>[2x]MIDYTAAGFTLLQGAH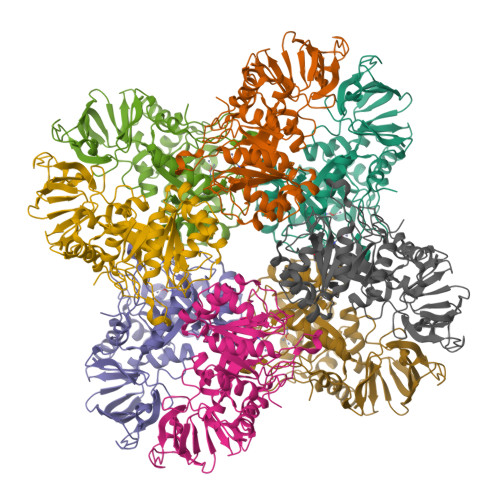LYAPEDRGICDVLVANGKIIAVASNIPSDIVPNCTVVDLSGQILCPGFIDQHVHLIGGGGQAGPTTRTPEVALSRLTEAGVTSVVGLLGTDSISRHPESLLAKTRALNEEGISAWMLTGAYHVPSRTITGSVEKDVAIIDRVIGVKCAISDHRSAAPDVYHLANMAAESRVGGLLGGKPGVTVFHMGDSKKALQPIYDLLENCDVPISKLLPTHVNRNVPLFEQALEFARKGGTIDITSSIDEPVAPAEGIARAVQAGIPLARVTLSSDGNGSQPFFDDEGNLTHIGVAGFETLLETVQVLVKDYDFSISDALRPLTSSVAGFLNLTGKGEILPGNDADLLVMTPELRIEQVYARGKLMVKDGKACVKGTFETA> MEVCLPNGHQIVDLINNAFEGRVSIYSAQEGWDKTISAQPDMMVCGGAVVCMHCLGV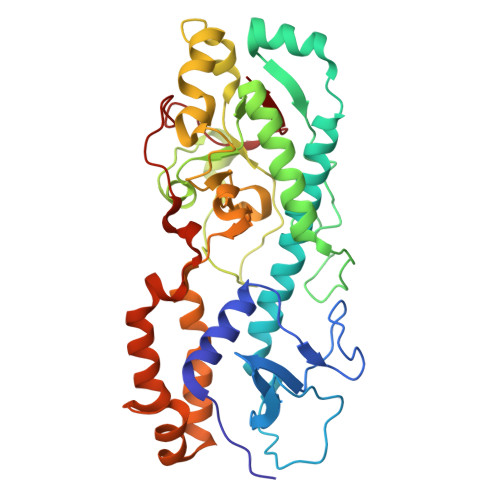VGSLQRKLKHLPHHRCNQQIRHQDYVDVQFADRVTAHWKRGMLSFVCQMHAMMNDVSPEDLDRVRTEGGSLVELNWLQVDPNSMFRSIHSSWTDPLQVVDDLDTKLDQYWTALNLMIDSSDLVPNFMMRDPSHAFNGVRLEGDARQTQFSRTFDSRSSLEWGVMVYDYSELEHDPSKGRAYRKELVTPARDFGHFGLSHYSRATTPILGKMPAVFSGMLTGNCKMYPFIKGTAKLKTVRKLVDSVNHAWGVEKIRYALGPGGMTGWYNRTMQQAPIVLTPAALTMFSDTTKFGDLDYPVMIGDPMILG> MAETREGGQSGAASILGAEAFPELLSKVPLNPQMDEDKH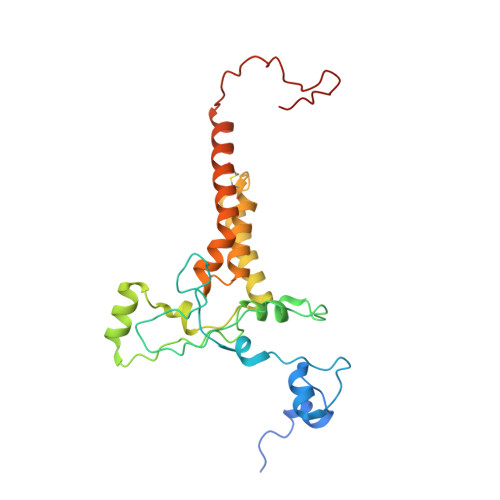FNKYKWGNEPIPVNRRTGSRMNSSIYDNRNHEAVRHPWSTDARTFHPNDNPEADRINTQYSNMVSDSFPEGGFSDAPRFSSNWERLLAYHHGLYSPEKFNSTTKTADEIRLAVNDFAAKVHADDPKNACKYLMIEEFKCLQSAQARIDPQGAATKCVKWFNEWRQCAWDQEKMVKGYNYIEDRRARKHKPYIGAPDLQYS3-deoxy-5-O-phosphono-beta-D-ribofuranose | C5 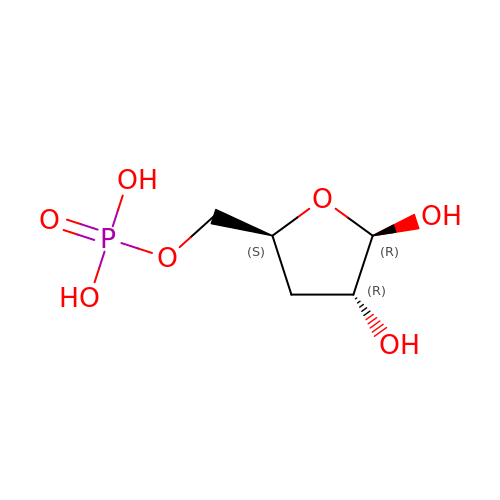H11 O7 P | OOLHLHJSMUTTHE-VPENINKCSA-N Complex I couples the transfer of two electrons from NADH to ubiquinone (Q) with the translocation of four protons across the membrane. The L-shaped complex is structured into a peripheral arm that protrudes into the aqueous milieu and catalyzes electron transfer with one FMN and 8–10 iron–sulfur ([Fe–S]) clusters, and a membrane arm embedded in the lipid bilayer that mediates proton translocation. We have determined structures of the electron-input module of complex I from the hyperthermophilic bacterium Aquifex aeolicus, encompassing subunits NuoE and NuoF that contain the FMN cofactor, the [4Fe–4S] cluster N3, and the [2Fe–2S] cluster N1a, respectively, both in the air-oxidized and dithionite-reduced states at resolutions up to 1.8 Å. Here, we show that the redox state of N1a regulates NADH oxidation in complex I by inducing a conformational change close to the NADH-binding site.

We therefore sought to lock the peptide bond in place by exchanging a nearby residue, G129E, with serine and aspartate, respectively. The longer side chains were intended to occupy the position of the bound water molecule that has to make way for the flipping peptide bond according to our structures. Thus, while both mutations fixed the position of the peptide bond, the Gly/Asp exchange seemed to exert a much stronger effect than the Gly/Ser mutation. Thus, fixing the flip of the peptide bond of E95F leads to a slower dissociation of NAD+ from the enzyme further decreasing the rate of the NADH/ferricyanide oxidoreductase activity.

>MFKTEFEFPEELKTKLQEHINYFPKKRQAILLCLHEIQNYYGYIPPESLKPLADMLELPLNHVEGVVAFYDMFDREDKAKYRIRVCVSIVCHLMGTNKLLKALENILGIKPGEVTPDGKFKIVPVQCLSACSEAPVFMVNDDEYKFESEVQLNEILSRYT[2x];>[2x]MRSYPAIPRIYAETTLNMLLKRAKKPRVHSIDEYLKDGGYQALEKALNMSPEEIIDWVDKSTLRGRGGAGFPTGKKWKFAVQNPGPRYFICNADESEPGTFKDRIIIERDPHLLIEGIIISSYAIGANEAYIYIRGEYPAGYYILRDAIEEAKKKGFLGKNILGSGFDLEIYVARGAGAYICGEETALIESLEGKRGHPRLKPPYPVQKGLWGKPTVVNNVETIANVPFIISMGWEEYRYIGPSDYAGPKLFPVSGKVKKPGVYELPMNTTLREVIFKYAGGTLGNKKVKAVFSGALDCFSSEELDIPMDYSPLGFGGTGTVIVLTEEDDIVEAALKIAEFYEHETCGQCTPCRVGCYEQANLLEKIYKGEATEQDWEGFDFVNRNIQPTSICGLGAVAGRLIRQTLEKFPEEWEKYRKKSASLPLAGHHHHHH> GAHVSRVEKLPKDYQ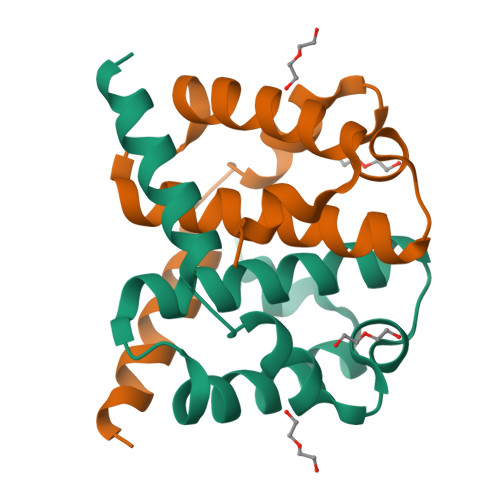IVYKEIQKYLFKVGPVELNEGIGLLSEILGFFEEGAAAGKGVLDVTGTDVAAFCDALIGDSKTYADLYQESIQQHVDKAMKNMKD> LEAELHNCVVVQFDGPMSFYVQMESDVPALEQMTDKLLDAEQDLPAFSDLKEGALCVAQFPEDEVFYRAQIRKVLDDGKCEVHFIDFGNNAVTQQFRQLPEELAKPARYSRHCELD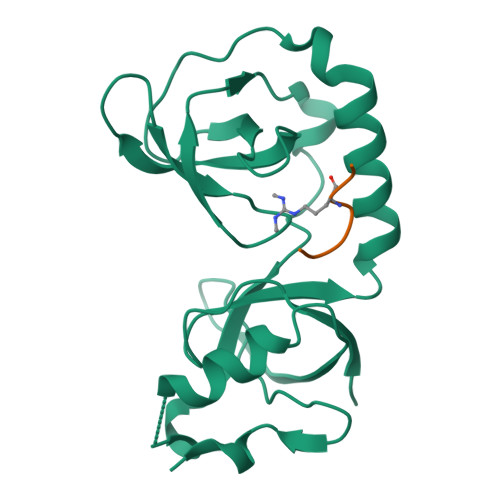ASTISKCDAALLQSFIDTRFSETFQVEILATKGTGTHVVRLFYQSKNISEKLQECQ;> NPVIARGRGRGRK>[2x]GSHMASPAAVNLGTAGNFVILAKSGISTTGTTHVTGDIGVSPITATGITGFGLTMDSSNTFATSALVTGKVYAADYTPPT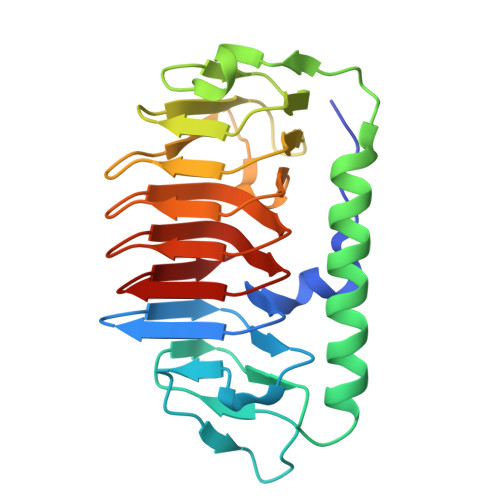PANMSTAVSDMETAYTAAAGVTAPAPVVELGAGNIGGMTLAPGVYKWSTGVTIPTDVTLAGGANDVWIFQIAQTLDLSNGIHVNLSGGAQAANIFWQVAGQTTLGTTSVFNGNILDQTAIVLNTGATLNGRALAQTAVTLDASTVSAS>[4x]MVRFSRDMLQDGAKRMFKWLRKGEGLPNYLIMYD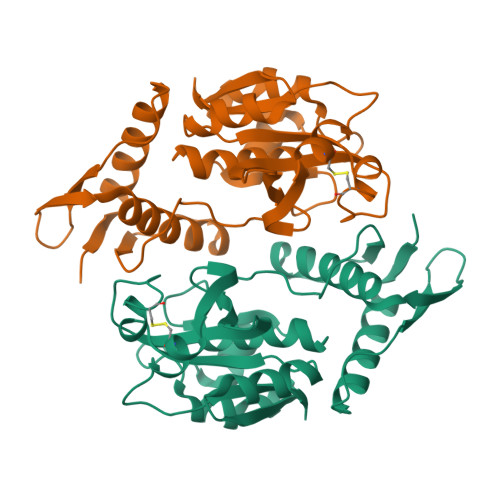MDRNKEYKLVPKEYAGLYESRNIFWIKNGREPNYVTLTSVARNPLVMDYQNTNYTACPTSLSLASQMLYHYKSESECAKALGTSKGSGTSPAQLIANAPKLGFKIIPIKRDSKEVKKYLKKGFPVICHWQVNQSRNCKGDYTGNFGHYGLIWDMTSTHYVVADPAKGVNRKYKFSCLDNANKGYRQNYYVVCPA>[2x]GAMGGPKPGGGPGLSTPGGHPKPPHRGGGEPRGGRQHHPPYHQQHHQGPPPGGPGGRSEEKISDSEGFKANLSLLRRPGEKTYTQRCRLFVGNLPADITEDEFKRLFAKYGEPGEVFINKGKGFGFIKLESRALAEIAKAELDDTPMRGRQLRVRFATHAAALSVRNLSPYVSNE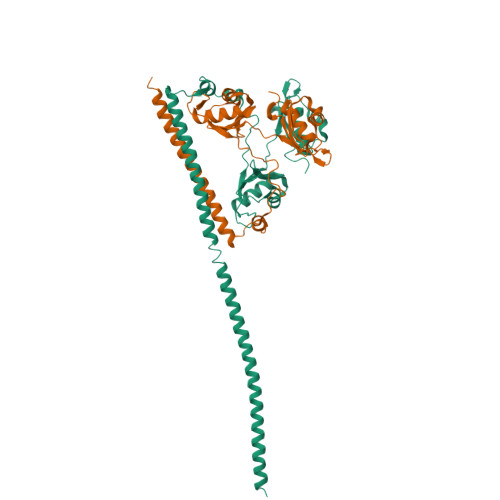LLEEAFSQFGPIERAVVIVDDRGRSTGKGIVEFASKPAARKAFERCSEGVFLLTTTPRPVIVEPLEQLDDEDGLPEKLAQKNPMYQKERETPPRFAQHGTFEYEYSQRWKSLDEMEKQQREQVEKNMKDAKDKLESEMEDAYHEHQANLLRQDLMRRQEELRRMEELHNQEMQKRKEMQLRQEEERRRREEEMMIRQREMEEQMRRQREESYS;>[2x]MEGLTIDLKNFRKPGEKTFTQRSRLFVGNLPPDITEEEMRKLFEKYGKAGEVFIHKDKGFGFIRLETRTLAEIAKVELDNMPLRGKQLRVRFACHSASLTVRNLPQYVSNELLEEAFSVFGQVERAVVIVDDRGRPSGKGIVEFSGKPAARKALDRCSEGSFLLTTFPRPVTVEPMDQLDDEEGLPEKLVIKNQQFHKEREQPPRFAQPGSFEYEYAMRWKALIEMEKQQQDQVDRNIKEAREKLEMEMEAARHEHQVMLM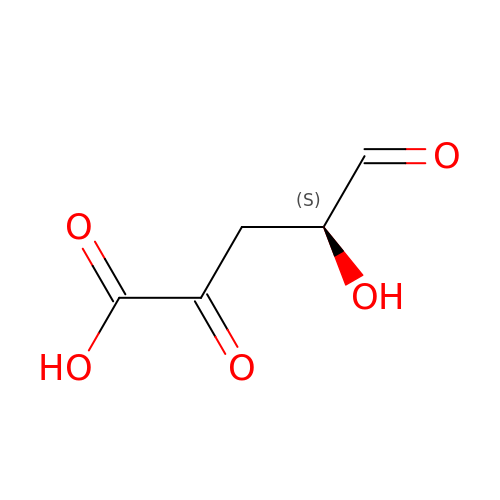(4S)-4-hydroxy-2,5-dioxopentanoic acid | C5 H6 O5 | QZKCWTOLHHFWCD-VKHMYHEASA-N> MEELDALLEE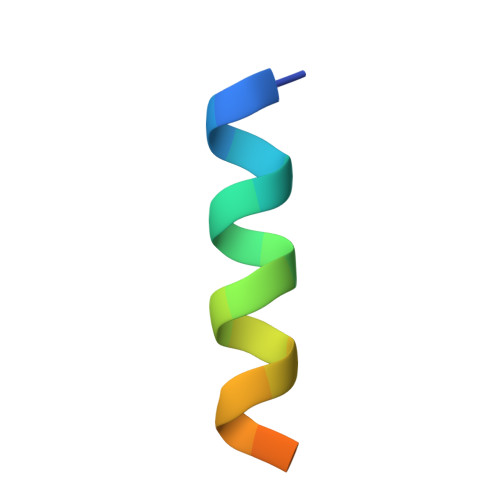LERSTLQDSD>HHHHHHSSGLVPRGSHMQTTTVYSLEDLLPYLKQDNVDVKLAPGTYNVNGFDVGEDRLFSTTPLFLFEGSNSTYDFTDVKLNINTVVLTKFGNNEVNEIQILGNNNVLKNLKLEDIGTTAPSNRAQSIVIDGRDNRIEGFHLTIRGSYPYGYGDAFGKGGGSVINHRKHSGVLIRGLRNHLKDCTIISRSYGHIVFMQAASYPTVEGCYIEGEMRSTDDMLAEEGTGSPADKVDFMTVWGYKLPAGYMMSLQEGGIAAYNAGTTYIDGVEIQ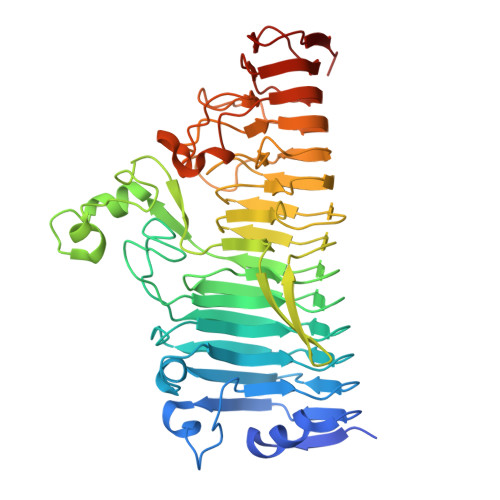RATDNPTVLNCTIKNARTGVTLAHANGTKYVEGCTVLGCENGYSIGSGTVVNCGADAIYGPVFKNTYGSDKGYNADITILPPSDAYYNGHDAVAYIGGSNHNLTFRSEITEIPSNLKIMVSGDLQGLRVLHGSNPSQNNFAGTNIVLRNLTNFPVDLHSDSSNITVTSCDTDNITDNGTNNSIEAIDCDSD[2x]> GRSTADSRRCPPGYFRMGRMRQCSRWLSCEELRTEVRQLKRVGEGAVKRVFLSEWKEHKVALSRLTRLEMKEDFLHGLQMLKSLQSEHVVTLVGYCEEDGTILTEYHPLGSLSNLEETLQLSKYQDVNTWQHRLQLAMEYVSIINYLHHSPLGTRVMCDSNDLPKTLSQYLLTSNFSIVANDLDALPLVDHDSGVLIKCGHRELHGDFVAPEQLWPYGEDTPFQDDLMPSYNEKVDIWKIPDVSSFLLGHVEGSDMVRFHLFDIHKACKSQIPAERPTAQNVLDAYQRVFHSLRDTVMSQTKEM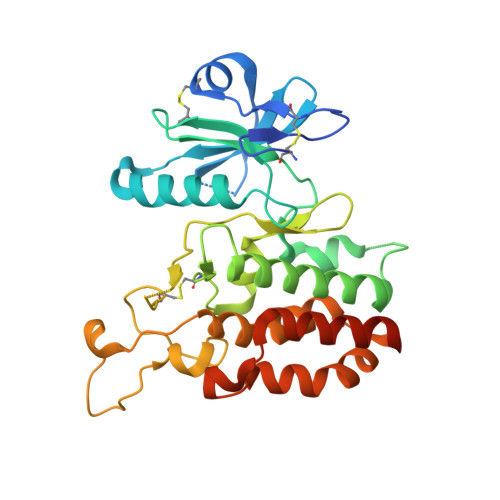L2-amino-9-{5-O-[(R)-{[(S)-{dichloro[(R)-hydroxy(phosphonooxy)phosphoryl]methyl}(hydroxy)phosphoryl]oxy}(hydroxy)phosphoryl]-2-O-methyl-beta-D-ribofuranosyl}-7-methyl-9H-purin-7-ium-6-olate 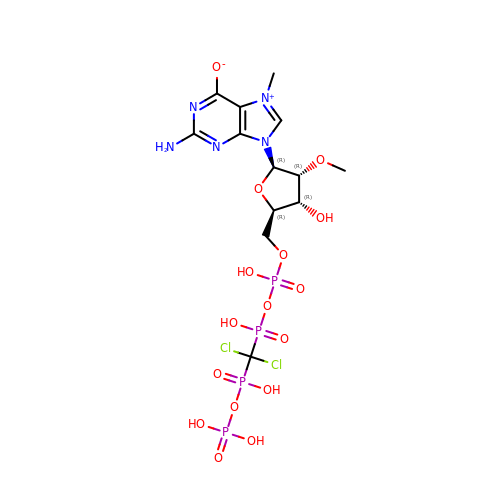| C13 H21 Cl2 N5 O16 P4 | ULCNCADMRQHHSX-IOSLPCCCSA-N>HMMSQQPPLRGSGDLGVLIERADGSVQILDGTAKTSLARVEGLGDLSHASLVFSRDQRYAYVFGRDGGLTKLDLLAQRIDKRLIQGGNSIGGAISQDGRLVAVSNYEPGGVKVFDSRTLELVAEIPATRLPGQDRNSRVVGLVDAPGQRFVFSLFDSGEIWIADFSQGDTPHLTRFRDIGKQPYDALISPDGRYYMAGLFGEDGMAQLDLWHPERGVRRVLGDYGRGQRKLPVYKMPHLEGWTIASDQAFVPAVGHHQVLVLDARDWKQTDAIDVAGQPVFVMTRPDDRQIWVNFAYPDNDKVQVIDSETHEVIETLRPGPGVLHMEFSGRGDQVWISVRDADQLQVWDPYRLKRIGSLPARSPSGIFFS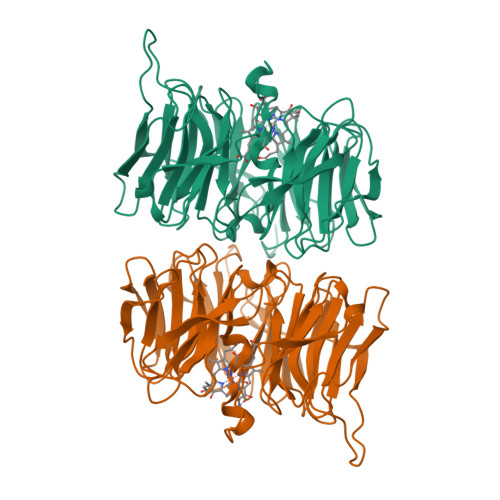HRAQHIGL[8x]> MQFSKMHGLGNDFVVVDGVTQNVFFTPETIRRLANRHCGIGFDQLLIVEAPYDPELDFHYRIFNADGSEVSQCGNGARCFARFVTLKGLTNKKDISVSTQKGNMVLTVKD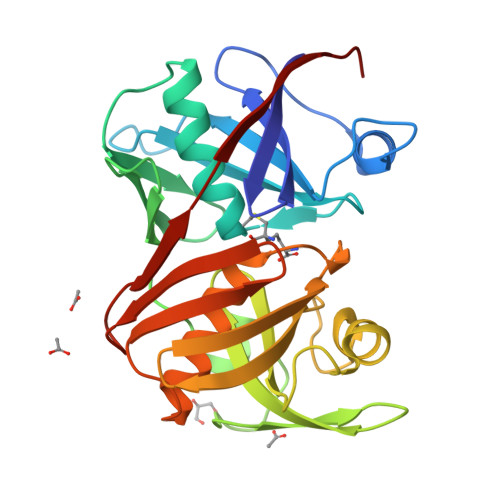DNQIRVNMGEPIWEPAKIPFTANKFEKNYILRTDIQTVLCGAVSMGNPHCVVQVDDIQTANVEQLGPLLESHERFPERVNAGFMQIINKEHIKLRVYERGAGETQACGSGACAAVAVGIMQGLLNNNVQVDLPGGSLMIEWNGVGHPLYMTGEATHIYDGFITL N-carbamimidoyl-2-[2-(2-chlorophenyl)-5-[4-(4-ethanoylphenoxy)phenyl]pyrrol-1-yl]ethanamide | C27 H23 Cl N4 O3 | 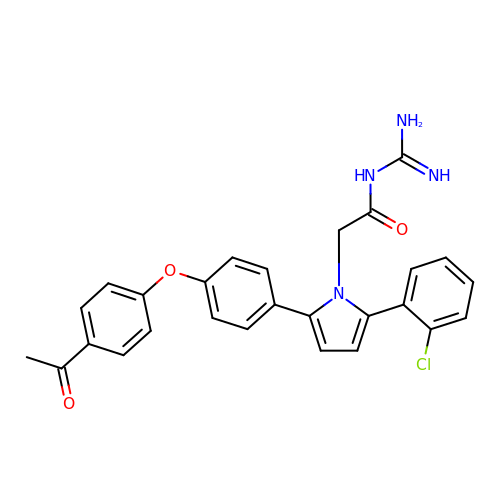MIEKBLPHNQZVQQ-UHFFFAOYSA-N>TNQCTVRYNVADCSHLKLTHIPDDLPSNITVLNLTHNQLRRLPPTNFTRYSQLAILDAGFNSISKLEPELCQILPLLKVLNLQHNELSQISDQTFVFCTNLTELDLMSNSIHKIKSNPFKNQKNLIKLDLSHNGLSSTKLGTGVQLENLQELLLAKNKILALRSEELEFLGNSSLRKLDLSSNPLKEFSPGCFQTIGKLFALLLNNAQLNPHLTEKLCWELSNTSIQNLSLANNQLLATSESTFSGLKWTNLTQLDLSYNNLHDVGNGSFSYLPSLRYLSLEYNNIQRLSPRSFYGLSNLRYLSLKRAFTKQSVSLASHPNIDDFSFQWLKYLEYLNMDDNNIPSTKSNTFTGLVSLKYLSLSKTFTSLQTLTNETFVSLAHSPLLTLNLTKNHISKIANGTFSWLGQLRILDLGLNEIEQKLSGQEWRGLRNIFEIYLSYNKYLQLSTSSFALVPSLQRLMLRRVALKNVDISPSPFRPLRNLTILDLSNNNIANINEDLLEGLENLEILDFQHNNLARLWKRANPGGPVNFLK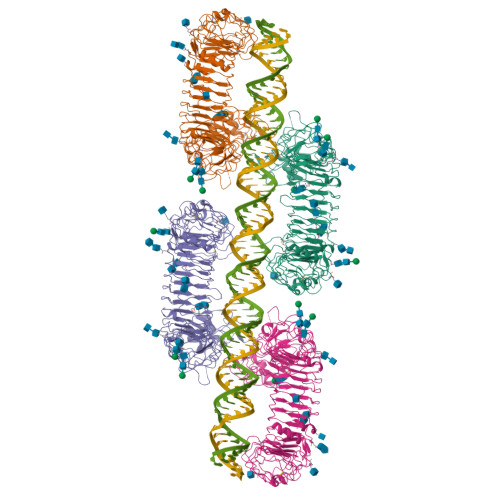GLSHLHILNLESNGLDEIPVGVFKNLFELKSINLGLNNLNKLEPFIFDDQTSLRSLNLQKNLITSVEKDVFGPPFQNLNSLDMRFNPFDCTCESISWFVNWINQTHTNISELSTHYLCNTPHHYYGFPLKLFDTSSCKDSAPFEL[4x]> GARARQENGMPEKPPGPRSPQREPQRVSHEQFRAALQLVVDPGDPRSYLDNFIK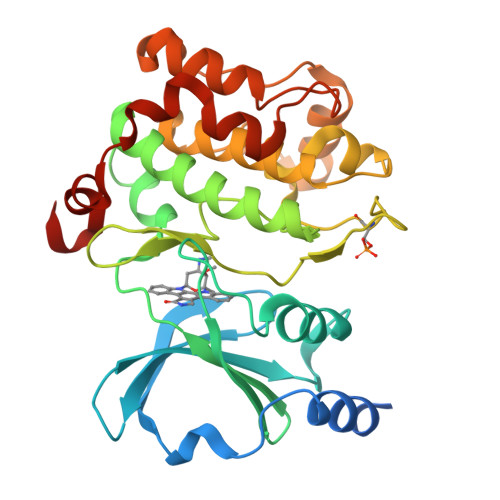IGEGSTGIVCIATVRSSGKLVAVKKMDLRKQQRRELLFNEVVIMRDYQHENVVEMYNSYLVGDELWVVMEFLEGGALTDIVTHTRMNEEQIAAVCLAVLQALSVLHAQGVIHRDIKSDSILLTHDGRVKLSDFGFCAQVSKEVPRRKSLVGTPYWMAPELISRLPYGPEVDIWSLGIMVIEMVDGEPPYFNEPPLKAMKMIRDNLPPRLKNLHKVSPSLKGFLDRLLVRDPAQRATAAELLKHPFLAKAGPPASIVPLMRQNRTR> SMSSAIKSYKSVLRPNERKNQLLKSTIQCLEDGSAFFFKMLQGLFGGITPEIVRFSTEQEKQQQDIALWCAVNWFRPVSQDSLTHTIASDNLVEKFEEYYGGTASDAIKQYFSASIGESYYWNDCRQQYYDLCRELGVEVSDLTHDLEILCREKCLAVATESNQNNSIISVLFGTGEKEDRSVKLRITKKILEAISNLKEIPKNVAPIQEIILNVAKATKETFRQVYAGNLGAPSTLEKFIAKDGQKEFDLKKLQTDLKKVIRGKSKERDWCCQEELRSYVEQNTIQYDLWAWGEMFNKAHTALKIKSTRNYNFAKQRLEQFKEIQSLNNLLVVKKLNDFFDSEFFSGEETYTICVHHLGGKDLSKLYKAWEDDPADPENAIVVLCDDLKNNFKKEPIRNILRYIFTIRQECSAQDILAAAKYNQQLDRYKSQKANPSVLGNQGFTWTNAVILPEKAQRNDRPNSLDLRIWLYLKLRHPDGRWKKHHIPFYDTRFFQEIYAAGNSPVDTCQFRTPRFGYHLPKLTDQT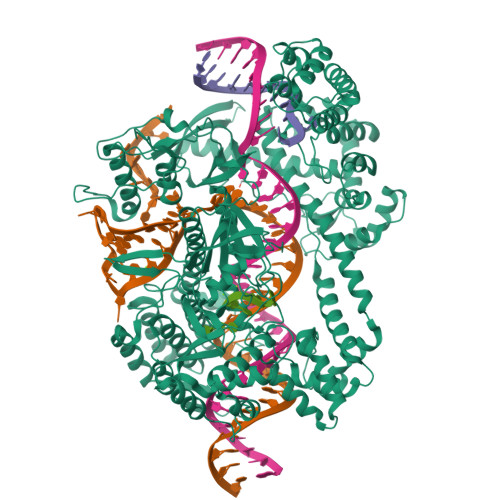AIRVNKKHVKAAKTEARIRLAIQQGTLPVSNLKITEISATINSKGQVRIPVKFDVGRQKGTLQIGDRFCGYDQNQTASHAYSLWEVVKEGQYHKELGCFVRFISSGDIVSITENRGNQFDQLSYEGLAYPQYADWRKKASKFVSLWQITKKNKKKEIVTVEAKEKFDAICKYQPRLYKFNKEYAYLLRDIVRGKSLVELQQIRQEIFRFIEQDCGVTRLGSLSLSTLETVKAVKGIIYSYFSTALNASKNNPISDEQRKEFDPELFALLEKLELIRTRKKKQKVERIANSLIQTCLENNIKFIRGEGDLSTTNNATKKKANSRSMDWLARGVFNKIRQLAPMHNITLFGCGSLYTSHQDPLVHRNPDKAMKCRWAAIPVKDIGDWVLRKLSQNLRAKNIGTGEYYHQGVKEFLSHYELQDLEEELLKWRSDRKSNIPCWVLQNRLAEKLGNKEAVVYIPVRGGRIYFATHKVATGAVSIVFDQKQVWVCNADHVAAANIALTVKGIGEQSSDEENPDGSRIKLQLTS>[2x]HHHHHHSSGLVPRGSHMTDLNIPHTHAHLVDAFQALGIRAGQALMLHASVKAVGAVMGGPNV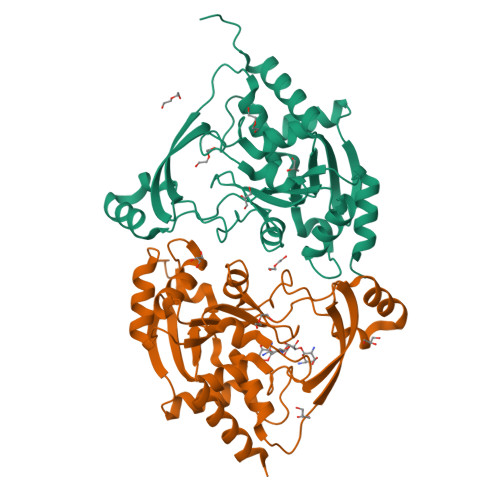ILQALMDALTPDGTLMMYAGWQDIPDFIDSLPDALKAVYLEQHPPFDPATARAVRENSVLAEFLRTWPCVHRSANPEASMVAVGRQAALLTANHALDYGYGVESPLAKLVAIEGYVLMLGAPLDTITLLHHAEYLAKMRHKNVVRYPCPILRDGRKVWVTVEDYDTGDPHDDYSFEQIARDYVAQGGGTRGKVGDADAYLFAAQDLTRFAVQWLESRFGDSASYG2-{[(benzyloxy)carbonyl]amino}-2-deoxy-beta-D-glucopyranose 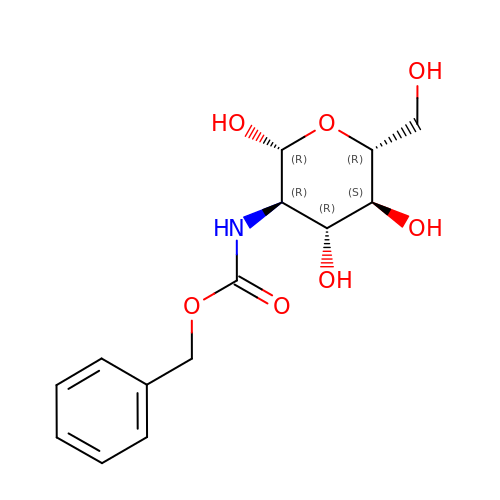| C14 H19 N O7 | FRTOTMQAWIIMKK-SYLRKERUSA-N> GNKICQFKLVLLGESRVGKSSLVLRFVKGQFHEFQESTIGAAFLTQTVCLDDTTVKFEIWDTAGQ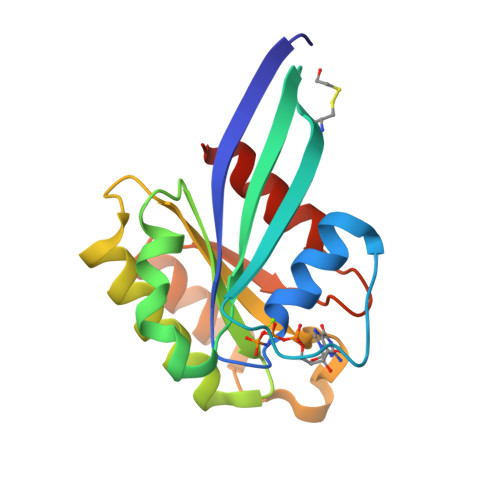ERYHSLAPMYYRGAQAAIVVYDITNEESFARAKNWVKELQRQASPNIVIALSGNKADLANKRAVDFQEAQSYADDNSLLFMETSAKTSMNVNEIFMAIAKKLPKN>[4x]MGLSLPKEKGLILCLWSKFCRWFQRRESWAQSRDEQNLLQQKRIWESPLLLAAKDNDVQALNKLLKYEDCKVHQRGAMGETALHIAALYDNLEAAMVLMEAAPELVFEPMTSELYEGQTALHIAVVNQNMNLVRALLARRASVSARATGTAFRRSPCNLIYFGEHPLSFAACVNSEEIVRLLIEHGADIRAQDSLGNTVLHILILQPNKTFACQMYNLLLSYDRHGDHLQPLDLVPNHQGLTPFKLAGVEGNTVMFQHLMQKRKHTQWTYGPLTSTLYDLTEIDSSGDEQSLLELIITTKKREARQILDQTPVKELVSLKWKRYGRPYFCMLGAIYLLYIICFTMCCIYRPLKPRTNNRTSPRDNTLLQQKLLQEAYMTPKDDIRLVGELVTVIGAIIILLVEVPDIFRMGVTRFFGQTILGGPFHVLIITYAFMVLVTMVMRLISASGEVVPMSFALVLGWCNVMYFARGFQMLGPFTIMIQKMIFGDLMRFCWLMAVVILGFASAFYIIFQTEDPEELGHFYDYPMALFSTFELFLTIIDGPANYNVDLPFMYSITYAAFAIIATLLMLNLLIAMMGDTHWRVAHERDELWRAQIVATTVMLERKLPRCLWPRSGICGREYGLGDRWFLRVEDRQDLNRQRIQRYAQAFHTRGSEDLDKDSVEKLVPRGSAAAWSHPQFEK

TRPV6 is a calcium-selective ion channel implicated in epithelial Ca2+ uptake. TRPV6 is a representative of the vanilloid subfamily of transient receptor potential (TRP) channels that is considered the principal epithelial calcium channel for Ca2+ absorption in intestines and many other organs. The channel is assembled of four subunits and contains two main components: a TMD with a central ion channel pore and an intracellular skirt that is mostly built of ankyrin repeat domains connected to each other by three-stranded β-sheets, N-terminal helices, and C-terminal hooks. The TMD is composed of six transmembrane helices S1–S6 and a re-entrant pore loop (P-loop) between S5 and S6.

As a control, we aimed to determine the open (apo) state structure of human TRPV6 (TRPV6Open) at a higher resolution than that of the previously solved structures. Initially, we improved the structural resolution for hTRPV6-CtD purified in glyco-diosgenin (GDN) detergent from 3.26 Å49 to 2.69 Å. The new open-state structures have the same architecture as previously published TRPV6 structures. Consistent with previous findings, the pore of the open-state TRPV6 was in the conducting state. Typical for the open conformation of TRPV6, S6 was not entirely α-helical and contained a π-bulge resulting from an α-to-π transition in its middle.[(1S,5R)-8-methyl-8-azabicyclo[3.2.1]octan-3-yl] (2S)-3-hydroxy-2-phenylpropanoate 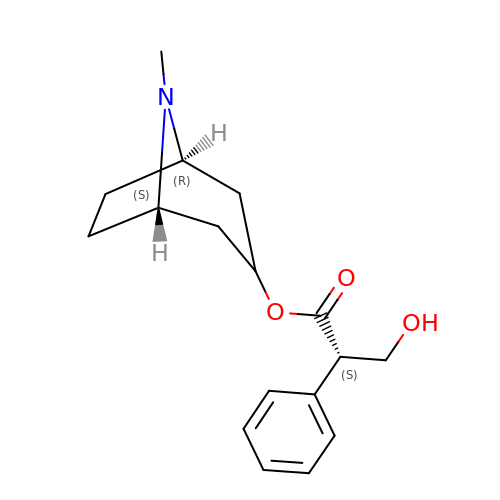| C17 H23 N O3 | RKUNBYITZUJHSG-FXUDXRNXSA-N> MIEKSQACHDSLLDSVGQTPMVQLHQLFPKHEVFAKLEYMNPGGSMKDRPAKYIIEHGIKHGLITENTHLIESTSGNLGIALAMIAKIKGLKLTCVVDPKISPTNLKIIKSYGANVEMVEEPDAHGGYLMTRIAKVQELLATIDDAYWINQYANELNWQSHYHGAGTEIVETIKQPIDYFVAPVSTTG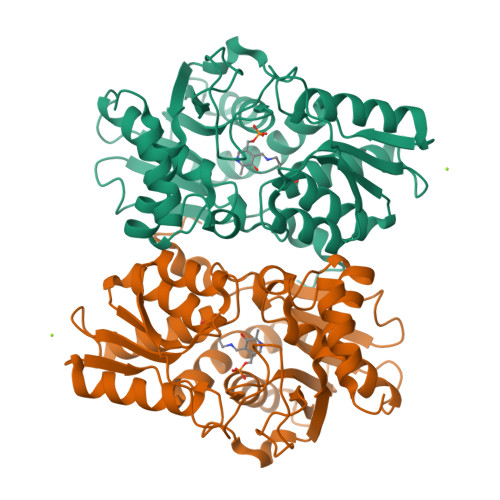SIMGMSRKIKEVHPNAQIVAVDAKGSVIFGDKPINRELPGIGASRVPEILNRSEINQVIHVDDYQSALGCRKLIDYEGIFAGGSTGSIIAAIEQLITSIEEGATIVTILPDRGDRYLDLVYSDTWLEKMKSRQGVKSE>[2x]MDVVSLDKPFMYFEEIDNELDYEPESANEVAKKLPYQGQLKLLLGE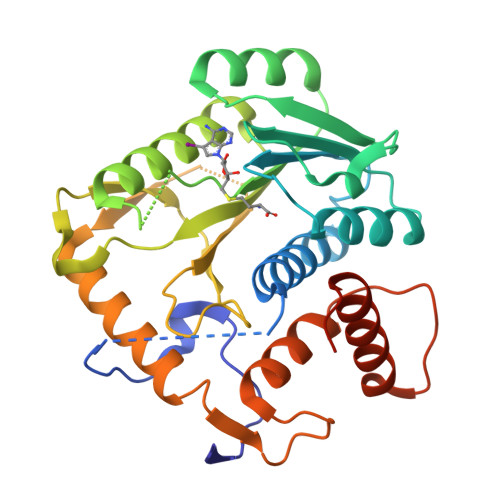LFFLSKLQRHGILDGATVVYIGSAPGTHIRYLRDHFYNLGVIIKWMLIDGRHHDPILNGLRDVTLVTRFVDEEYLRSIKKQLHPSKIILISDVRSKRGGNEPSTADLLSNYALQNVMISILNPVASSLKWRCPFPDQWIKDFYIPHGNKMLQPFAPSYSAEMRLLSIYTGENMRLTRVTKSDAVNYEKKMYYLNKIVRNKVVINFDYPNQEYDYFHMYFMLRTVYCNKTFPTTKAKILFLQQSIFRFLNIPTTSTEKVSHE>TVLPGVEAIGLGYNPFISYASVNSGAVQLFDWATAKKREVPFKAGYFVPEIVDVQQNDSATYTNVSGNTISEYQRSLATSVAIEGRYNFFSGSLSTDFDSNSLRNAENEFTRIQQSINLWSLRLPSVKSLRELMLPHMRQQLDELNVNDPKAISRYFDRVGSHFLTGIVMGGRAILASSTNKLRVKRDYSVSVVAKASYEGLTGQLSAEAKAKYGESISSFTQYSNTHQEVRGGDGAKAHGVFSGKKEDFQAWVDSVSASPDFVDFVPTIPMQEIWTLCSSEAQAEAMRKHYDDVWAPAQSEKYRVKANYIDQLVVITGGSSTIEPPVGYSKIEYDLNAGAGGDFIYLCYHEQTWQADRPKDAVTDIRIIFNKEPTPPGYTKLPQDLNKGAGGDDVFLCYKTEAYNTDTAINKVTVIGGNNADINAPYGYLKVPGDLNRGAGGNFIYACTFVGK[21x]

Mpf2Ba1 is a 53.2 kDa protein isolated from Pseudomonas monteilii through a multi-step purification process informed by artificial diet bioactivity screening against WCR larvae. The protein is comprised of two domains—an N-terminal MACPF domain and a C-terminal β-prism domain. Pore-forming proteins (PFPs) are a major class of soluble proteins that oligomerize into rings and undergo large irreversible conformational changes to become transmembrane assemblies and breach the membrane of target cells. We have identified and characterized the non-Bt insecticidal protein Mpf2Ba1, providing mechanistic details for how it effectively kills the devastating maize pest WCR by forming pores in midgut membranes targeting a different binding site than the insecticidal proteins currently deployed in commercial transgenic maize hybrids.

We were able to convert Mpf2Ba1 pre-pores into pores by either introducing lipids, in the form of POPC and 4% cholesterol mixed liposomes, or by raising the incubation temperature between ~50–53 °C without adding lipids. Although heating is not the physiological trigger, it appears to catalyze the refolding of the α-helical TMHs into β-hairpins to form a β-barrel, which has higher thermal stability than the helical conformation, confirming that pre-pore-to-pore conversion is endothermic. The 2D classes of the pore showed a distribution of stoichiometries, ranging from 21- to 24-fold, demonstrating heterogeneity of oligomerization. It was also evident that Mpf2Ba1 pores dimerized tail-to-tail: the barrel of one pore was inserted inside the other, and the inner and outer pore had different stoichiometries (3D classes in red and blue). Despite the most common stoichiometry in the 2D classes being a 22-mer, the inner ring of each dimer showed a consistent 21-fold symmetry and a clear structure, while the outer ring was a mixture of 22-fold and higher symmetries. Therefore, we decided to refine the 3D structure of the inner 21-mer pore, which was determined at 2.6 Å resolution and revealed a pore with an outer diameter of 240 Å, β-barrel diameter of 135 Å, and a height of 120 Å, increased by 40 Å from the pre-pore conformation. In the pore conformation, the β-sheet at the MACPF core straightens by an average dihedral angle of 36° to allow the helical bundles to refold into membrane-spanning β-hairpins and collectively form a β-barrel. The straightening of the MACPF central β-sheet repositions the HTH, which is pushed ~8 Å towards the lumen of the pore, restricting the diameter locally from 135 to 110 Å. This shift brings the HTH in close lateral contact with residues of the neighboring subunit, where Phe273 contacts Tyr92 on β1-strand in a π-π interaction, and the side-chain nitrogen of His270 forms a H-bond with the oxygen of Gln145 on β2-strand.> MFNQRTKNGVKKILAITAASTVFSMFGSSISIIEAASAPGVYVTPKNSVSSDIISIDWSPVQTAPYTYWAVHNWNQGGEAGGYAGFQQQSGFDENGKRTLHFAVWDPISSKEAIKAEYVSPTSVASNFGGEGTGLKIQTTYDWKNYNWYRMTMRSWQENGHTKFGQWLKDVSKNQWKLIGIMDFPVPNVTFNYGQTLFQEDWLGNGQDVREARVKNGYGRNISDKKWTSWNTQSIEGQEPLNNNWDGGATSEYLWFKAGGDSRSTIGTGKTFTLNQPSQPEIGKLDYDVKSTYYENEKLNITWQLKDSSTPQFKGKIEIYNNENMTGQPINVINDIKSYQNGISQSISLPTNTYAKIVLTDIFDQTVEKKVKIKNESPNILEGDRFAWSMKGIGDFEFAKLDLNKSTEELQVSLIAGTPHNYFDSTYASIKVQDTSGKVVYNKEIYGNTQ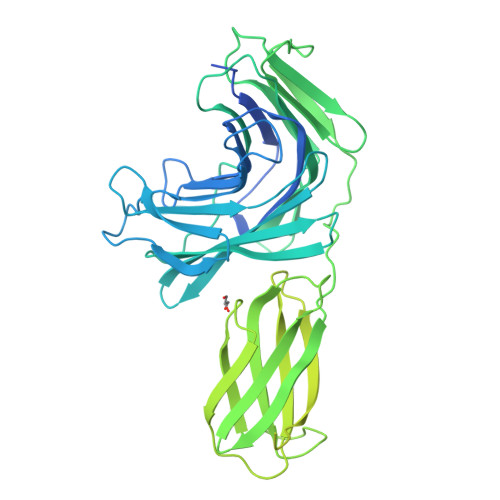QNAESKTVPVKVGNFIELTHLEGGERATLTNLDNNKRESFDKKVIYEVTKDGLKKINQIVNPKPDTEAPTQPQGLYASNVASDSVELKWNPSTDNVGVKEYQVLRDGQLIQTVQETKVTDQNLTANKEYKYTVKAVDTAGNISVQSNILTVTTKSQNVTYEKWDPKKAYTKGDKVEYQGKFYEAVQSYQGNGDPTWIFALSLWQPFKLI>MKKLLEELETKKTTIEEERNEITQRIGELKNKIGDLKTAIEELKKAKGKCPVCGRELTDEHREELLSKYHLDL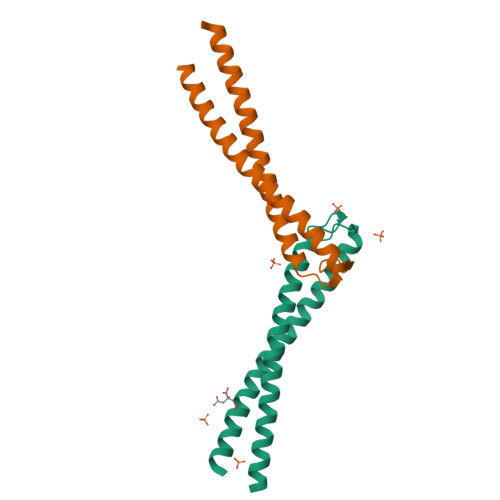NNSKNTLAKLIDRKSELERELRRIDMEIKRLTPLLTVAE[2x]> ELTQSRVQKIWVPVNSPTVIVMVGLPARGKTYISKKLTRYLNWIGVPTKVFNVGEYRREAVKQYSSYNFFRPDNEEAMKVRKQCALAALRDVKSYLAKEGGQIAVFDATNTTRERRHMILH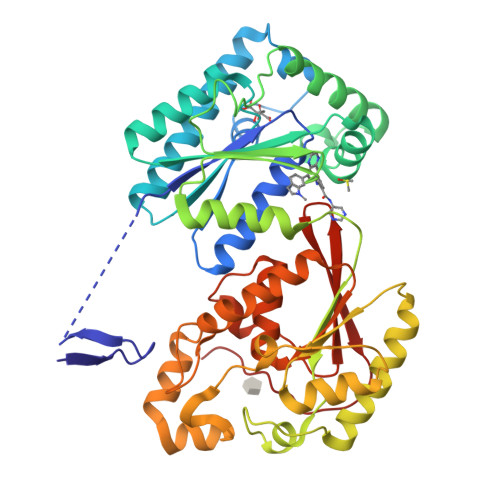FAKENDFKAFFIESVCDDPTVVASNIMEVKISSPDYKDCNSAEAMDDFMKRISCYEASYQPLDPDKCDRDLSLIKVIDVGRRFLVNRVQDHIQSRIVYYLMNIHVQPRTIYLCRHGENEHNLQGRIGGDSGLSSRGKKFASALSKFVEEQNLKDLRVWTSQLKSTIQTAEALRLPYEQWKALNEIDAGVCEELTYEEIRDTYPEEYALREQDKYYYRYPTGESYQDLVQRLEPVIMELERQENVLVICHQAVLRCLLAYFLDKSAEEMPYLKCPLHTVLKLTPVAYGCRVESIYLNVESVCTHRERS GH19 chitinase hydrolyzes the glycosidic bonds of chitin, namely beta-1, 4-linked N-acetyl-D-glucosamine. One of the physiological roles of chitinase is to defend plants against pathogenic fungi by degrading chitin, a major component of the cell wall of many fungi. By revealing the evolutionary history and loops appearance of GH19 chitinase, we discover that one loop which is remote from the catalytic site, is necessary to acquire the new antifungal activity. We demonstrate that this remote loop directly accesses the fungal cell wall, and surprisingly, it needs to adopt a defined structure supported by long-range intramolecular interactions to perform its function.

To investigate the contribution to the antifungal activity of the 45 substitutions, we constructed mutants of Anc4 + Loop II with substitutions in proximity to loop II. We chose six substitutions within 4.0 Å from Loop II and introduced them accordingly to their proximity to each other’s (Fig. 4C, D: mutations A, p12K and n13H; mutation B, s58T mutations C, n193G, y194F, and d197R). Two substitutions, p12K and n13H (small and large character indicates Anc4 and Anc5 state, respectively), formed new hydrogen bonding with Asp73 residue in loop II. The His 13 residue is also involved in hydrophobic interaction with Trp78 residue in loop II (upper left in the enlargement). d197(217)R (residue numbers are responsible to Anc5ΔLoop I; residue numbers in Anc5 state are in parentheses) substitution formed new hydrogen bonds between the N terminus and the tenth α-helix (upper right in the enlargement). n193(213)G substitution reduced structural hindrance with the Tyr76 residue in loop II (bottom left in the enlargement). Mutations A, B, and C increased antifungal activity 4.7, 1.2, and 5.4-fold, respectively. These substitutions increased antifungal activity while retaining the same degree of chitinase activity. MD simulations of these mutants revealed a gradual reduction of loop II flexibility directly related to the introduction of these six substitutions Furthermore, these substitutions decreased only the mobility of loop II not the one of a loop region between the ninth and tenth α-helices (positions 192–201). Furthermore, crystal structures of Anc4 + Loop II + A and Anc4 + Loop II + A + B + C revealed that their loop II structures are retained as in the structure of Anc5’s loop II, namely the antifungal active variant. Altogether, these results exemplify that antifungal activity enhanced by cell wall binding activity is supported by the substitutions that rigidify loop II.

> MVSRSMFDQLFKHRNSFYTYDAFIAAAKSFPSFGTTGDTDVRKREIAAFFAHVSHETSGGWPTAPDGPYAWGLVYIEEINQSNDYCDPSTQYPCAPGKQYYGRGPLQLSWNYNYGPCGDALGLDLLNNPDLVAQDPVIAFKTALWFWMTPQSPKPSCHDVMTGNWTPSSADLAAGRVPGFGVTTNIINGGLECGKGNPAQAENRVNYYKDFCNQLGVSPGSNLDCANMRPFG> PTFNKITPNLAEFAFSLYRQLAHQSNSTNILFSPVSIAAAFAMLSLGAKGDTHDEILEGLNFNLTEIPEAQIHEGFQELLRTLNQPDSQLQLTTGNGLFLSEGLKLVDKFLEDVKKLYHSEAFTVNFGDTEEAKKQINDYVEKGTQGKIVDLVKELDRDTVFALVNYIFFKGKWERPFEVKDTEEEDFHVDQVTTVKVPMMKRLGMFNIQHCKKLSSWVLLMKYLGNATAIFFLPDEGKLQHLENELTHDIITKFLENEDRRSASLHLPKLSITGTYDLKSVLGQLGITKVFSNGADLSGVTEEAPLKLSKAVHKAVLTIDEKGTEAAGA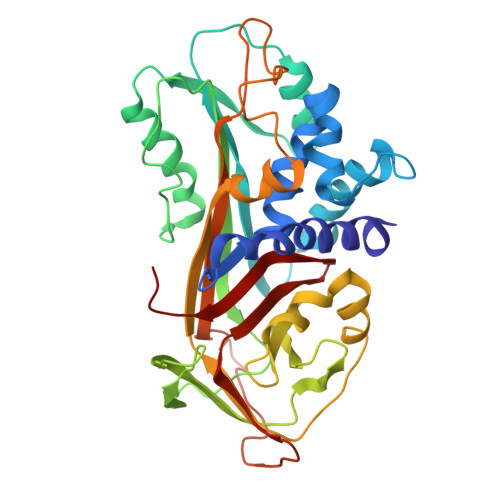MFLEAIPMSIPPEVKFNKPFVFLIIEQNTKAPLFMGRVVNPTQK> IVLEPIYWNSSNSKFLPGGGLVLYPQIGDKLDIICPKVDSKTVGQYEYYKVYMVDKDQADRCTIKKENTPLL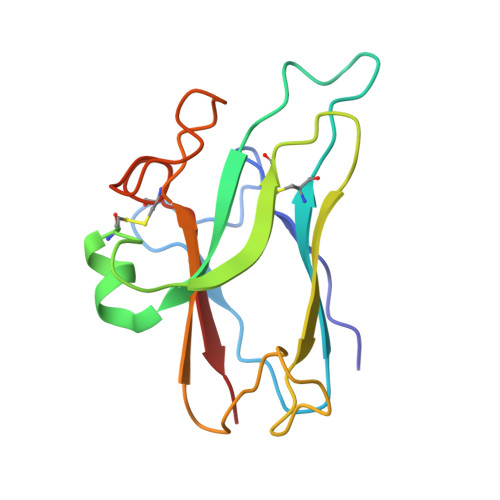NCARPDQDVKFTIKFQEFSPNLWGLEFQKNKDYYIISTSNGSLEGLDNQEGGVCQTRAMKILMKVG> QDEKPRYKDPSVPVEERVTDLLGRMTLEEKMSQLIQGDITNWMNETTGEFNLTGLEWSTKMRGGMFYVGYPVPWDYIADNVKKAQDYILQNTTLGIPAIVQTESLHGFLIGNATIYNSPIGFACSFNPELIEKMARLIGQEASALGVNHVMGPVVDLARELRFGRVEETYGEDPFLAGEIGYHYTKGIQSHNISANVKHFVGFSQPEQGLNTAPVHGGERYLRTTWLPSFKRAIMDAGAWSIMSAYHSYDGIPAVADYHTLTEILREEWGYKYWVTSDAGASDRVCTAFKLCRADPIDKEAVTLAILPAGNDVEMGGGSYNFETIIDLVNAGKLDIEIVNTAVSRVLRAKFEMGLFENPYNAAPASEWNKLIHTQEAVDLARELDRESIVLLENHDNALPLKKSGSIAVIGPMAHGFMNYGDYVVYESQYRGVTPLDGIKAAVGDKATINYAQGCERWSNDQSGFAE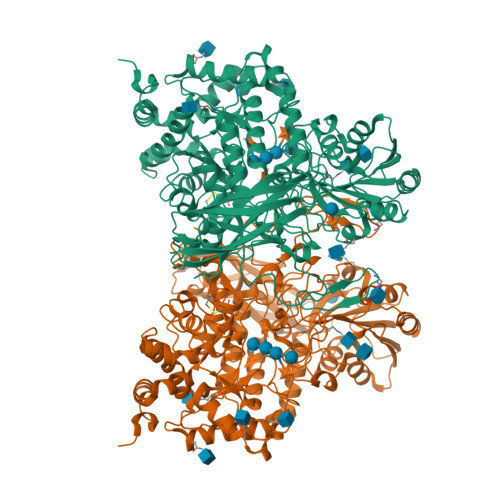AVEAAKKSDVAVVVVGTWSRDQKELWAGLNATTGAHVDVNSLSLVGAQAPLIKAIIDTGVPTVVVLSSGKPITEPWLSNNTAALVQQFYPSEQGGNALADVLFGDYNPSGKLSVSFPHSVGDLPIYYDYLNSAREIGDAGYIYSNGTLEFGHQYALGNPKAWYPFGYGKSYSSFEYGAVKLDKTNVTEADTVTVSVDVKNTDATREGTEVVQVYVVDEVASVVVPNRLLKGFKKVVIPAGQTKTVEIPLKVQDLGLWNVRMKYVVEPGAFGVLVGSSSEDIRGNATFYVQVDHHHHHH>[6x]MRGSHHHHHHGSSHANINAFKEAVTKIDRVEINRRLELAYAYNASIAGAKTNGEYPALKDPYSAEQKQAGVVEYARMLEVKEQIGHVI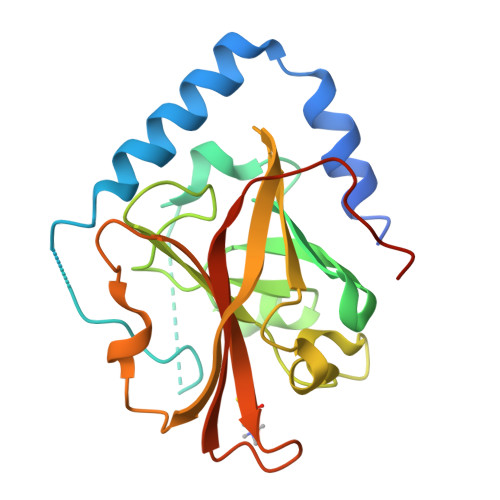IPRINQDIPIYAGSAEENLQRGVGHLEGTSLPVGGESTHAVLTAHRGLPTAKLFTNLDKVTVGDRFYIEHIGGKIAYQVDQIKVIAPDQLEDLYVIQGEDHVTLLTCTPYMINSHRLLVRGKRIPYVEKTVQKDSKTFRQQQ> MMNKRNWLLALSLSLAFSPCYADWAKLKAAASDLGAAVSETSKEVWQDVSDFSKKSWASISAWGEEAFNTAGVWTDKSIATGKEWLKAADKELNEMLNPKTAKEARIAINTMADTALIRLFNEQPSAKLLFDKAYGYAVFDSRKFSLMLHTNQGAGVAVNRKTGKHTYMKMFGAGLAAGIGGKFYQQVILFEDKARFDAFVT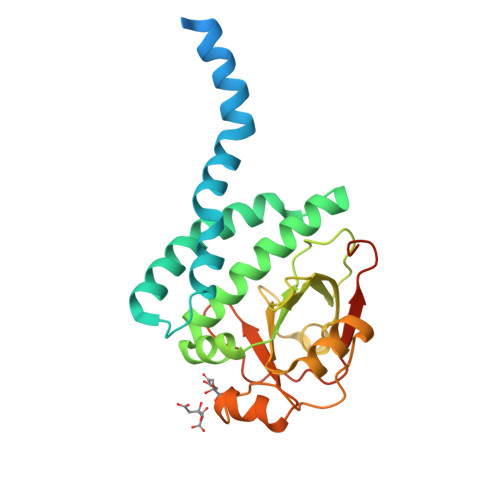QGWEATSEVGVVAGKESAELTAKYNGGMAIYQIGEKGLLLDANISGSKYWIDKDLTETSRLEHHHHHH>GNSQVFYLKYSKAEDLVDVLKQVSGTLTAAKEEAEGTVGSGREVVSIAASKHSNALIVTAPQDIMQSLQSVIEQLDIRRAQVHVEALIVEVAEGSNINFGVQWGSKDAGLMQFANGTQIPIGTLGAAISAAKPQKGSTVISENGATTINPDTNGDLSTLAQLLSGFSGTAVGVVKGDWMALVQAVKNDSSSNVLSTPSITTLDNQEAFFMVGQDVPVLTGSTVG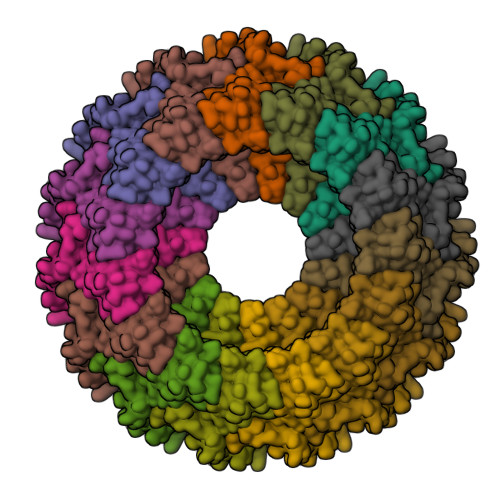SNNSNPFNTVERKKVGIMLKVTPQINEGNAVQMVIEQEVSKVEGQTSLDVVFGERKLKTTVLANDGELIVLGGLMDDQAGESVAKVPLLGDIPLIGNLFKSTADKKEKRNLMVFIRPTILRDGMAADGVSQRKYNYMRAEQIYRDEQGLSLMPHTAQPILPAQ[15x]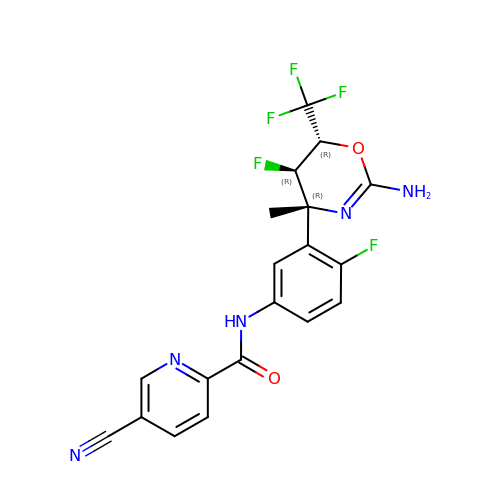N-{3-[(4R,5R,6R)-2-amino-5-fluoro-4-methyl-6-(trifluoromethyl)-5,6-dihydro-4H-1,3-oxazin-4-yl]-4-fluorophenyl}-5-cyanopyridine-2-carboxamide | C19 H14 F5 N5 O2 | UMHIFKHNODSZCU-HDMKZQKVSA-N4-({4-[(1S,4S)-5-(cyanoacetyl)-2,5-diazabicyclo[2.2.1]heptan-2-yl]pyrimidin-2-yl}amino)-N-ethylbenzamide 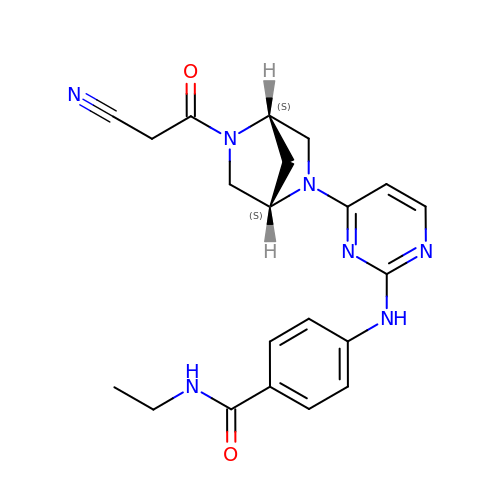| C21 H23 N7 O2 | YUJXKTRZTBIDCL-IRXDYDNUSA-N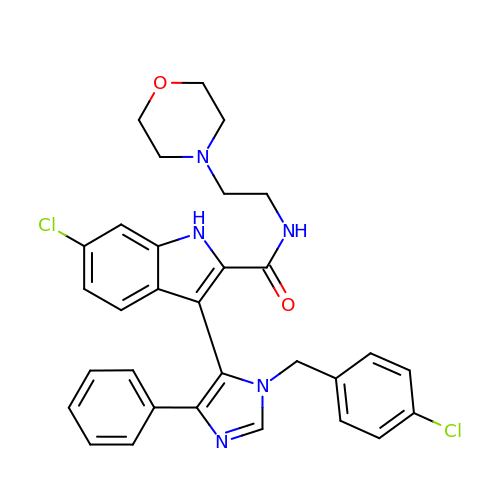6-chloro-3-[1-(4-chlorobenzyl)-4-phenyl-1H-imidazol-5-yl]-N-[2-(morpholin-4-yl)ethyl]-1H-indole-2-carboxamide | C31 H29 Cl2 N5 O2 | IFORBTVIRBZFON-UHFFFAOYSA-N>SNAGGSATGTGLVYVDAFTRFHCLWDASHPECPARVSTVMEMLETEGLLGRCVQVEARAVTEDELLLVHTKEYVELMKSTQNMTEEELKTLAEKYDSVYLHPGFFSSACLSVGSVLQLVDKVMTSQLRNGFSINRPPGHHAQADKMNGFCMFNNLAIAARYAQKRHRVQRVLIVDWDVHHGQGIQYIFEEDPSVLYFSVHRYEDGSFWPHLKESDSSSVGSGAGQGYNINLPWNKVGMESGDYITAFQQLLLPVAYEFQPQLVLVAAGFDAVIGDPKGGMQVSPECFSILTHMLKGVAQGRLVLALE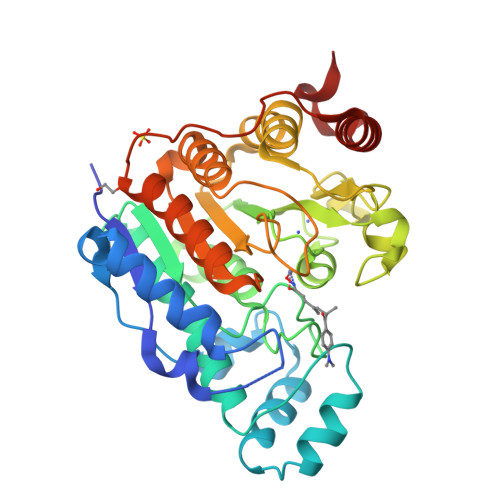GGYNLQSTAEGVCASMRSLLGDPCPHLPSSGAPCESALKSISKTISDLYPFWKSLQTFE[2x]> MANYPHTPTQAAKRRKETLMLQKLRNRKGFTLIELLIVVAIIGILAAIAIPQFSAYRVKAYNSAASSDLRNLKTALESA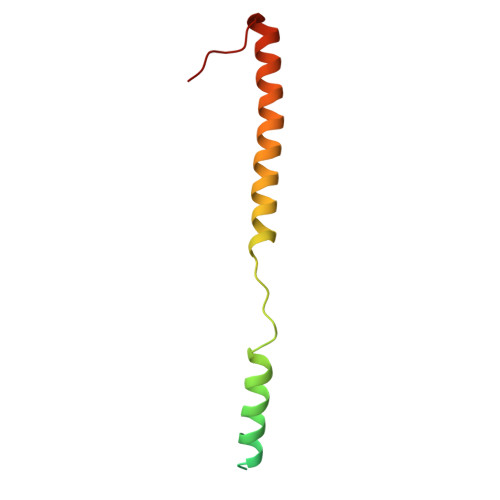FADDQTYPPES> GSSKLIHVPKEDNSKEVTLDSLLEEGVLDKEIHKAITRMEFPGLTPVQQKTIKPILSSEDHDVIA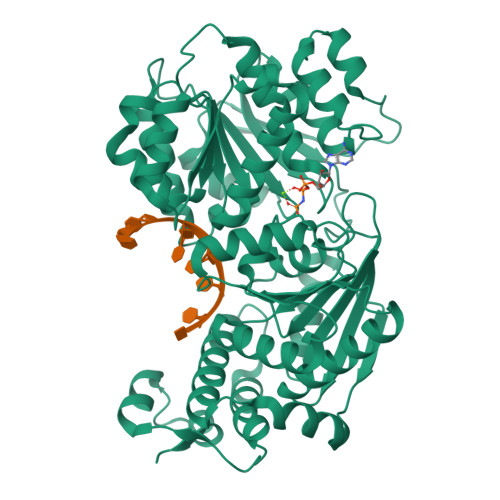RAKTGTGKTFAFLIPIFQHLINTKFDSQYMVKAVIVAPTRDLALQIEAEVKKIHDMNYGLKKYACVSLVGGTDFRAAMNKMNKLRPNIVIATPGRLIDVLEKYSNKFFRFVDYKVLDEADRLLEIGFRDDLETISGILNEKNSKSADNIKTLLFSATLDDKVQKLANNIMNKKECLFLDTVDKNEPEAHERIDQSVVISEKFANSIFAAVEHIKKQIKERDSNYKAIIFAPTVKFTSFLCSILKNEFKKDLPILEFHGKITQNKRTSLVKRFKKDESGILVCTDVGARGMDFPNVHEVLQIGVPSELANYIHRIGRTARSGKEGSSVLFICKDELPFVRELEDAKNIVIAKQEKYEPSEEIKSEVLEAVTEEPEDISDIVISLISSYRSCIKEYRFSERRILPEIASTYGVLLNDPQLKIPVSRRFLDKLGLSRSPIGKAMFEIRDY>HHHHHHLPNITILATGGTIAGGGDSATKSSYTVGKVGVENLVNAVPQLKDIANVKGEQVVNIGSQDMNDNVWLTLAKKINTDCDKTDGFVITHGTDTMEETAYFLDLTVKCDKPVVMVGAMRPSTS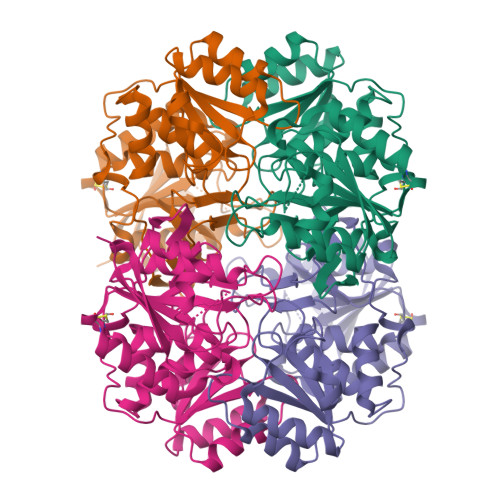MSADGPFNLYNAVVTAADKASANRGVLVVMNDTVLDGRDVTKTNTTDVATFKSVNYGPLGYIHNGKIDYQRTPARKHTSDTPFDVSKLNELPKVGIVYNYANASDLPAKALVDAGYDGIVSAGVGNGNLYKSVFDTLATAAKTGTAVVRSSRVPTGATTQDAEVDDAKYGFVASGTLNPQKARVLLQLALTQTKDPQQIQQIFNQY[4x]>[2x]SNAQVISETFSSGRLNRKQKIGIYKPEKYTDRQAYPLIVVLNAETLMEPVVSMVRYYEQFGEMPKCIVVGVYEPKQEDVTVVEEVGRPINESARFFEFVSAELVPYIQGKYPIADLKGV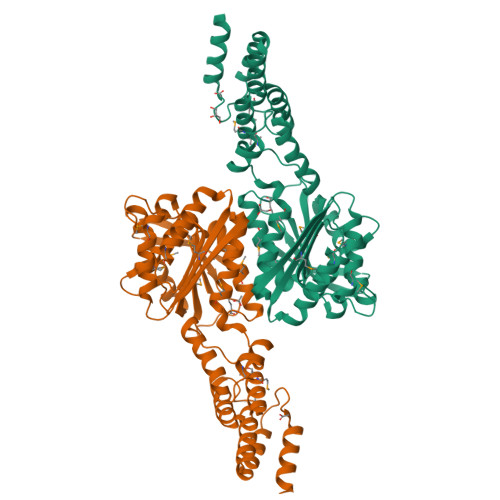IASEEAGFLANYYMLAEKKPTFNMIVSLNPVALPRMGEEFSHALAAGVPNRLFYYMATADVENKVVYDKAIQFERAMRSAPVHESVEYHFVDFKGSSVNAAKLQGIAQALDMCFDIYKPIGGKEFKTQMETLETGIYEYLENKYNTIYKQLGVKKVPILNDVMATYTAINSSQDWESLKKLAKYVESNGYLKTAMPNFFLAEYYEKIGDDKKALKTYQKAYTEPNIDFITGDLINERITHLQATKRKSKHTKVIEPIEPTEEVAPAQEEQNPTDESNQN> GENIVCRVICTTGQI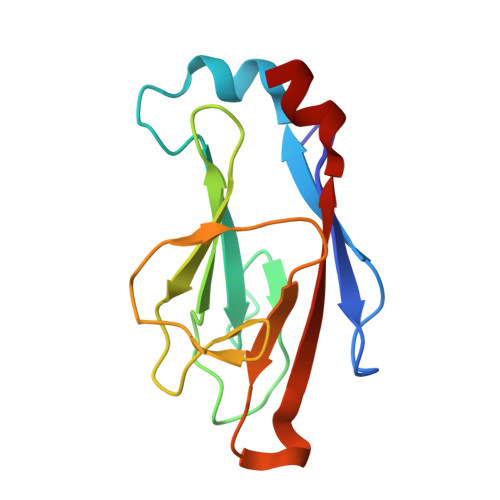PIRDLSADISQVLKEKRSIKKVWTFGRNPACDYHLGNISRLSNKHFQILLGEDGNLLLNDISTNGTWLNGQKVEKNSNQLLSQGDEITVGVGVESDILSLVIFINDKFKQCL>MVHWADYIADKIIRERGEKEKYVVESGITPSGYVHVGNFRELFTAYIVGHALRDKGYEVRHIHMWDDYDRFRKVPRNVPQEWKDYLGMPISEVPDPWGCHESYAEHFMRKFEEEVEKLGIEVDLLYASELYKRGEYSEEIRLAFEKRDKIMEILNKYREIAKQPPLPENWWPAMVYCPEHRREAEIIEWDGG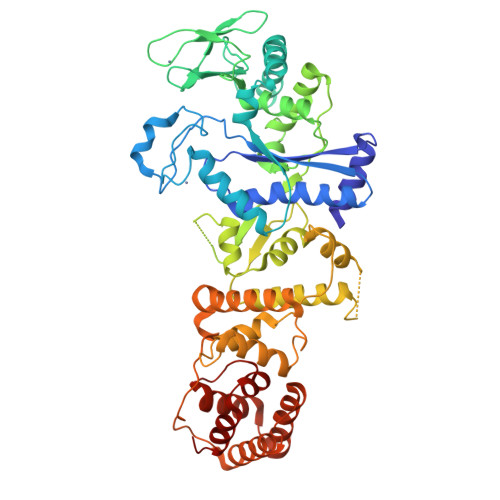WKVKYKCPEGHEGWVDIRSGNVKLRWRVDWPMRWSHFGVDFEPAGKDHLVAGSSYDTGKEIIKEVYGKEAPLSLMYEFVGIKGQKGKMSGSKGNVILLSDLYEVLEPGLVRFIYARHRPNKEIKIDLGLGILNLYDEFEKVERIYFGVEGGKGDDEELRRTYELSMPKKPERLVAQAPFRFLAVLVQLPHLTEEDIINVLIKQGHIPRDLSKEDVERVKLRINLARNWVKKYAPEDVKFSILEKPPEVEVSEDVREAMNEVAEWLENHEEFSVEEFNNILFEVAKRRGISSREWFSTLYRLFIGKERGPRLASFLASLDRSFVIKRLRLEG[2x]>MENTENSVDSKSIKNLEPKIIHGSESMDSGISLDNSYKMDYPEMGLCIIINNKNFHKSTGMTSRSGTDVDAANLRETFRNLKYEVRNKNDLTREEIVELMRDVSKEDHSKRSSFVCVLLSHGEEGIIFGTNGPVDLKKITNFFRGDRCRSLTGKPKLFIIQACRGTELDCGIETD[2x];>SGVDDDMACHKIPVEADFLYAYSTAPGYYSWRNSKDGSWFIQSLCAMLKQYADKLEFMHILTRVNRKVAAEFESFSFDATFHAKKQIPCIVSMLTKELYF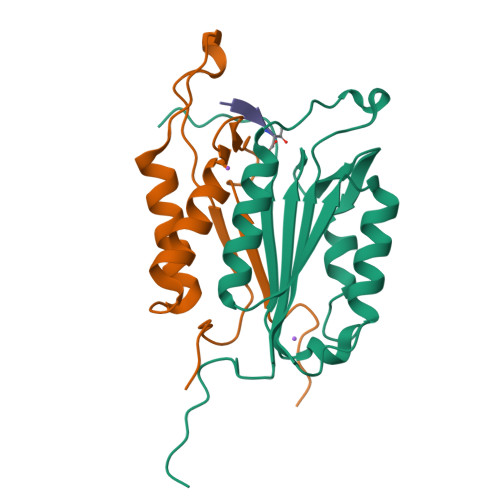YHH[2x]>[2x]MQDYTVHIVDDEEPVRKSLAFMLTMNGFAVKMHQSAEAFLAFAPDVRNGVLVTDLRMPDMSGVELLRNLGDLKINIPSIVITGHGDVPMAVEAMKAGAVDFIEKPFEDTVIIEAIERA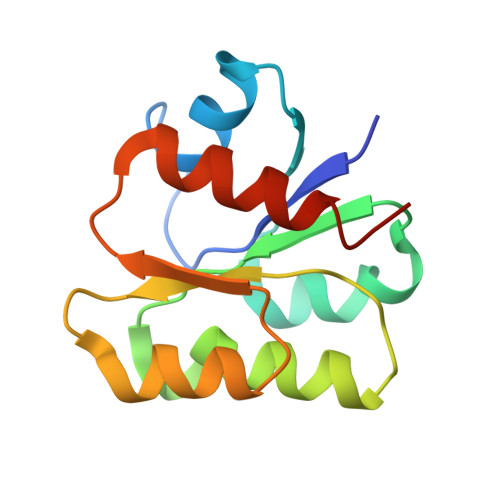SEHLVALE> SMSLLDAHIPQLIASEANFGAKAALMRSTIAQAEQAAMSSQAFHMGEASAAFQ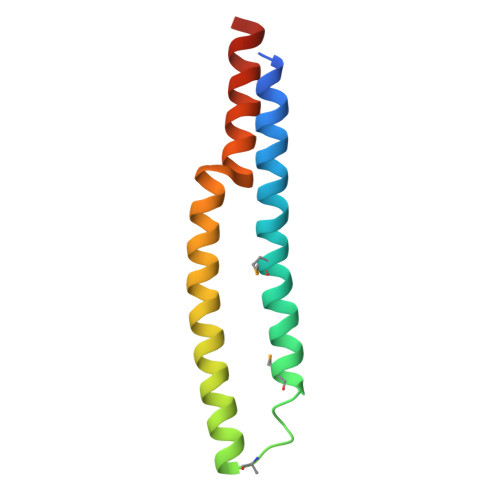AAHARFVEVSAKVNALLDIAQLNIGDAASSYVAQDAAAASTYTGI>MGLAVFLPPYPFRGLKAPYLWMFYKYLHCATDSILFITGEDYLSVTDDEAQRARWEFDPASMASLGYELPNAQSMACHEYLTLDNAFYETLLSRHHHDPIKSFSAFLTERIPDLETELHALLDSKKGIIDQIDTFISICNCPSLEHVARTLGKEVMHIEIGPLRAPMYRNTAYLDFAGVNGGTEASARYEKCQAEFDIKASLGDLHNYFLEVLPPAEAATHSAAGVVLQVEDNSNLIAYNHDFTNISLLSYVRQRYEKEDILVRAHPGSLFRL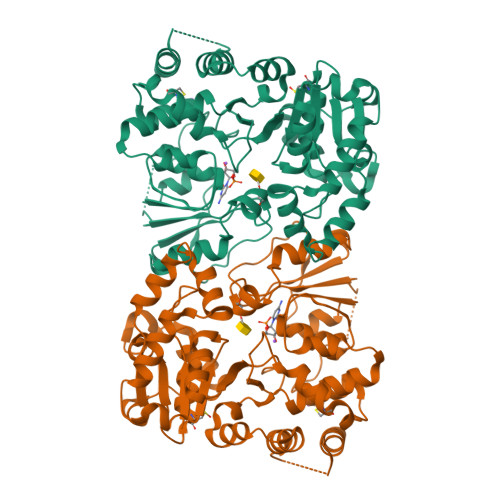RDDVFTIDDSANSLAFINQCNEVFTINSSVGLEAILTGKKTTVLGDCSYAFINELAGASATVNAAAFYLFSYLVPFDLVFNQEYLKFRLGHPEEREIVGKHIEFYSADMPGSLSQAAHSLSSLINEAISLEHHHHHH[2x]>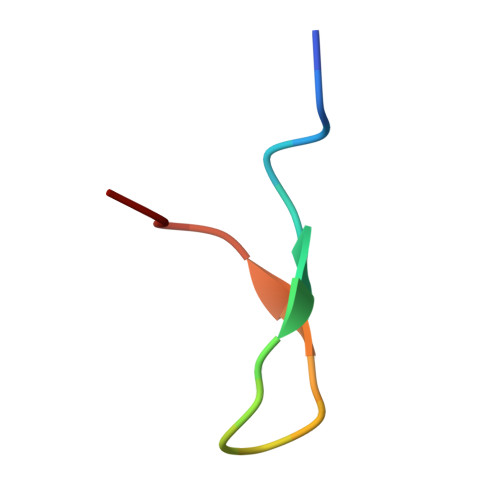 GPGSRGKSTVTGRMISGWL>MGLELFLDLVSQPSRAVYIFAKKNGIPLELRTVDLVKGQHKSKEFLQINSLGKLPTLKDGDFILTESSAILIYLSCKYQTPDHWYPSDLQARARVHEYLGWHADCIRGTFGIPLWVQVLGPLIGVQVPEEKVERNRTAMDQALQWLEDKFLGDRPFLAGQQVTLADLMALEELMQPVALGYELFEGRPRLAA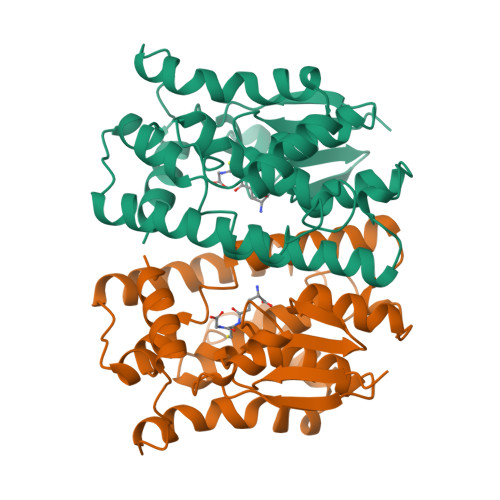WRGRVEAFLGAELCQEAHSIILSILEQAAKKTLPTPSPEAYQAMLLRIARIP[2x]> GSHMPPNRPGITFEIGARLEALDLLQK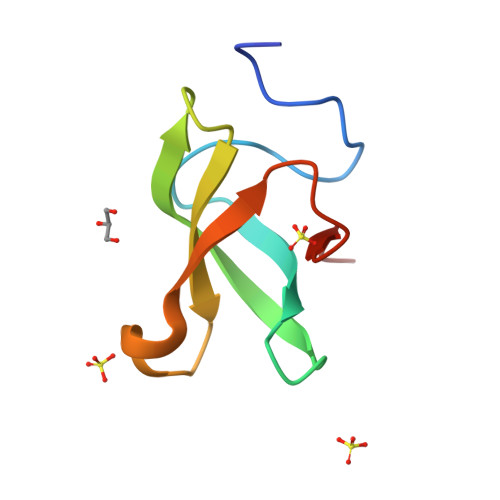WYPSRIEKIDYEEGKMLVHFERWSHRYDEWIYWDSNRLRPLER>MADNMTTTQIEVGPGATNATINFEAGILECYERFSWQRALDYPGQDRLHRLKRKLESRIKTHNKSEPENKRMSLEERKAIGVKMMKVLLFMDPSAGIEGFEPY[2x];>M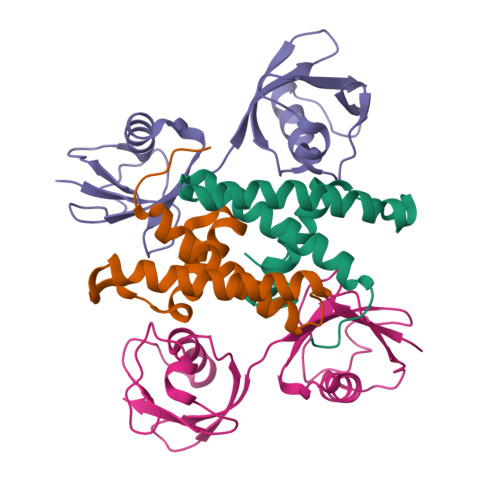GGDLTVKMLGGQEILVPLRDSMTVSELKQFIAQKINVPAFQQRLAHLDSREVLQEGVPLVLQGLRAGSTVLLVVQNSISILVRNDKGRSSPYEVQLKQTVAELKQQVCQKERVQADQFWLSFEGRPMDDEHPLEEYGLMKGCTVFMNLRLRGG[2x]>MAVYLCTCGTSAAKKFFGQTPRFDAAWVTEHGGVEAASKVIYDTFRTARLDDEVALKRDLSAEIHSLARMGVNDKDTVVLFSSETADGQACAWAVKRYLEQARPGILCRIEVVAGLQVTDAHVFRTAGVLNFTKAVLHEIDANGTGQCVLNPTGGFKSLVPYTVLIGMLRGVPAKYIFEQSSALIPLPMMPVEFARSRLEPLRPLLERIQNETAIPRAELDKALPSFEEREILDSLFEDVGQGQVSLSPVGFLIWEELERPTALVPFLSRRALDDLLKMRATEGTAPDDYITRVARSPEQLAIG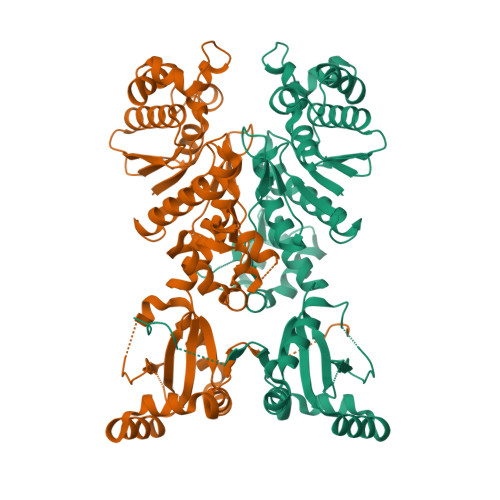KHESWSKGLFWLKRGEHTRDRYLVSVEGWRLLVWRIVDHDEYDDLLTQNRKTDAGARVVAERREKYAPFVRLELYEDGEGWSHPQFEKGVEGHHHHHHHHHH[2x]>GDITHMAPSRKFFVGGNWKMNGRKQSLGELIGTLNAAKVPADTEVVCAPPTAYIDFARQKLDPKIAVAAQNCYKVTNGAFTGEISPGMIKDCGATWVVLGHSERRHVFGESDELIGQKVAHA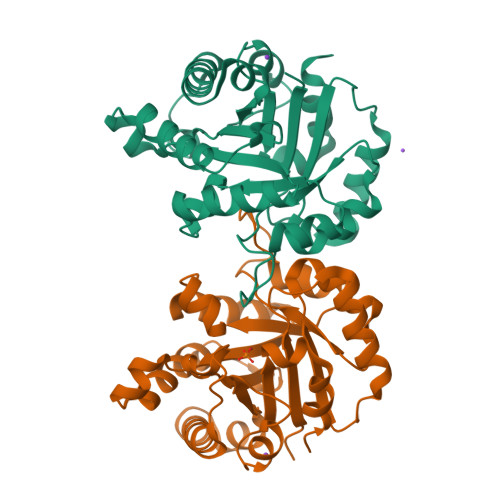LAEGLGVIACIGEKLDEREAGITEKVVFEQTKVIADNVKDWSKVVLAYEPVWAVGTGKTATPQQAQEVHEKLRGWLKSNVSDAVAQSTRIIYGGSVTGATCKELASQPDVDGFLVGGASLKPEFVDIINAKQ[2x]>[2x]CHAINAAGKKVLIVYAHQEPKSFNGSLKNVAVDELSRQGCTVTVSDLYAMNFEPRATDKDITGTLSNPEVFNYGVETHEAYKQRSLASDITDEQKKVREADLVIFQF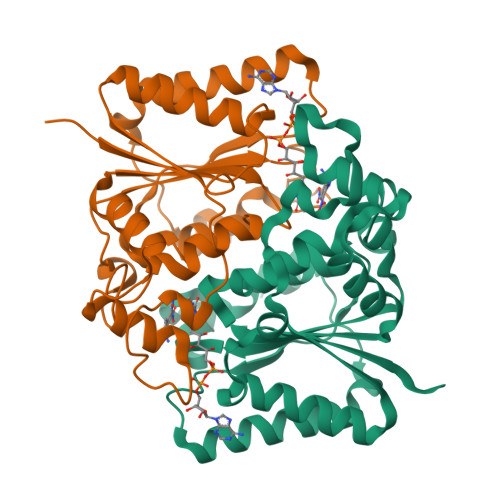PLYWFSVPAILKGWMDRVLCQGFAFDIPGFYDSGLLQGKLALLSVTTGGTAEMYTKTGVNGDSRYFLWPLQHGTLHFCGFKVLAPQISFAPEIASEEERKGMVAAWSQRLQTIWKEEPIPCTAHWHFGQ> MEFDDDLVDAEGNLVENGGTYYLLPHIWAHGGGIETAKTGNEPCPLTVVRSPNEVSKGEPIRISSQFLSLFIPRGSLVALGFANPPSCAASPWWTVVDSPQGPAVKLSQQKLPE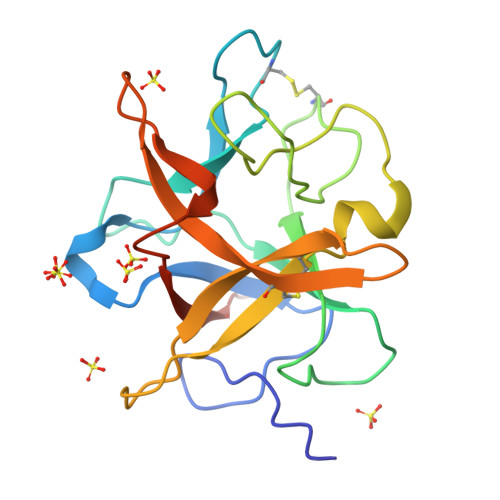KDILVFKFEKVSHSNIHVYKLLYCQHDEEDVKCDQYIGIHRDRNGNRRLVVTEENPLELVLLKAKSETASSH> MENTENSVASKSIKNLEPKIIHGSESMASGISLDNSYKMDYPEMGLCIIINNKNFHKSTGMTSRSGTDVDAANLRETFRNLKYEVRNKNDLTREEIVELMRDVSKE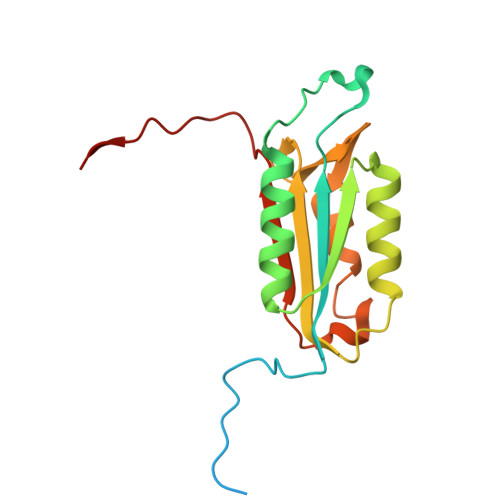DHSKRSSFVCVLLSHGEEGIIFGTNGPVDLKKITNFFRGDRCRSLDGKPKLFIIQACRGTELDCGIETD> XY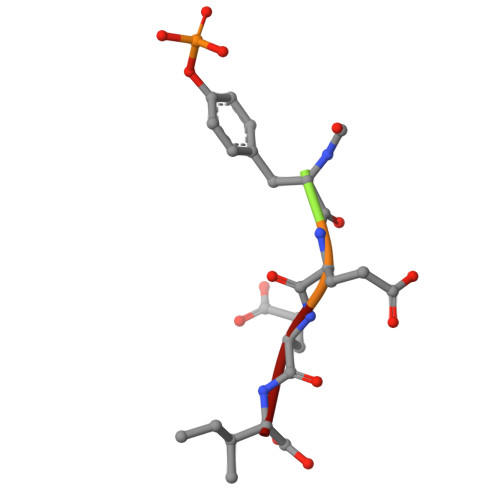EEI Members of the Hsp70 and Hsp40 (DnaJ-like) families function in specific pairs that form transient complexes with non-native regions of polypeptides to promote the folding, assembly and transport of proteins within the cell. All types of Hsp40 proteins contain a J-domain that can stimulate the ATPase activities of Hsp70. The human type II Hsp40 Hdj1 has been shown to function as a molecular chaperone to promote efficient protein folding. Hdj1 can bind to the non-native polypeptide and suppress the protein aggregation.

The crystal structure of the Hdj1 putative peptide-binding fragment was determined to 2.7Å resolution by the molecular replacement method using the Sis1 structure as the search model. The Hdj1 monomer structure contains domain I, II and the C-terminal dimerization motif. The two Hdj1 monomers are associated into a homo-dimer through the C-terminal dimerization motif. The Hdj1 homo-dimer forms a U-shaped architecture and a large cleft is formed between the two elongated monomers. When the domain II of Hdj11 is superimposed with that of the Sis1 structure, we found that the domain I of Hdj1 in the complex structure was kinked about 7.1° away from that in Sis1 structure. The domain re-arrangements within Hdj1 were achieved by the rotation of the linker region between domain I and domain II (residues 242 to 249). When we examined the peptide-binding site on the domain I of Hdj1 structure, several hydrophobic residues were identified to participate in forming the peptide-binding site. These residues include L168, M183, I185 and F237. In the Hdj1 structure, K181, K184 and K242 are well-positioned to interact with the EEVD motif from Hsp70. The peptide-binding site in the Hdj1 structure is not occupied by any amino acid residue, so the Hdj1 structure may represent the free Hsp40 state.

> KKQDPPVTHDLRVSLEEIYSGCTKKMKISHKRLNPDGKSIRNEDKILTIEVKKGWKEGTKITFPKEGDQTSNNIPADIVFVLKDKPHNIFKRDGSDVIYPARISLREALCGCTVNVPTLDGRTIPVVFKDVIRPGMRRKVPGEGLPLPKTPEKRGDLIIEFEVIFPERIPQTSRTVLEQVLPI>MKLSGGVEWALHCCVVLTAASRPVPAARLAELHDVSPSYLAKQMQALSRAGLVRSVQGKTGGYVLTRPAVEITLLDVVQAVDGPDPAFVCTEIRQRGPLATPPEKCTKACPIARAMGAAEAAWRASLAATTIADLVATVDDESGPDALP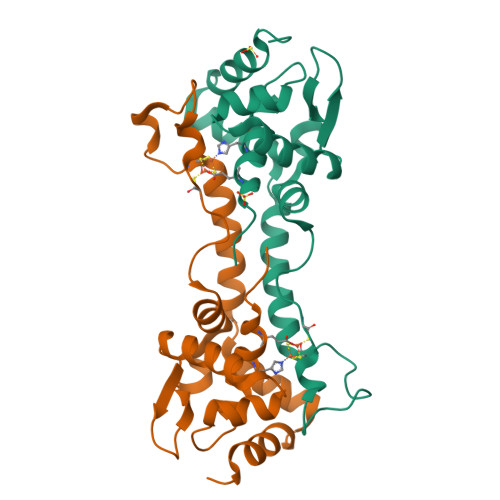GVGAWLIEGLGHHHHHH[4x]> CDATCQFRKAIDDCA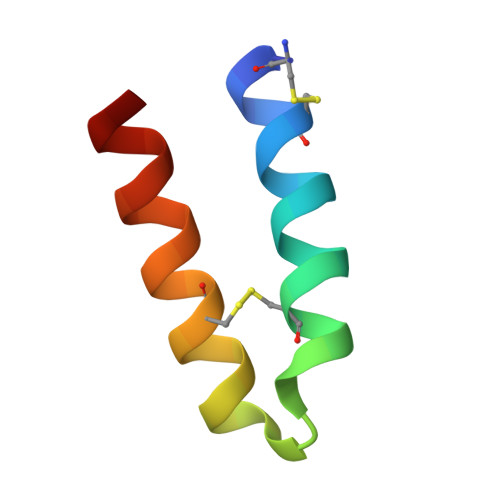RQAYHSSVFKACMKQKKKEWKAGX(2R,4S,5S)-5-amino-6-[4-(2-chlorophenyl)-2,2-dimethyl-5-oxopiperazin-1-yl]-2-ethyl-4-hydroxy-N-[(1R,2S,3S,5S,7S)-5-hydroxytricyclo[3.3.1.1~3,7~]dec-2-yl]hexanamide 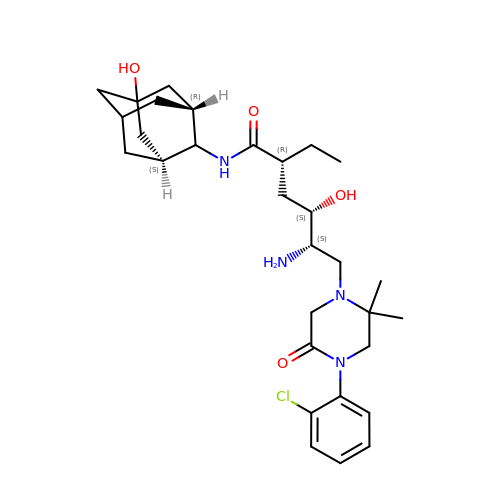| C30 H45 Cl N4 O4 | MGQQKSSUXHKDSK-PTMRNKDMSA-N> GSHMEAVQNRIVEAAERVPGVRGVIHLRARYVGQDIWADMIIGVDPENTVEQAEEICEAVQAAVCGKIRRIESLHVSAEAREIG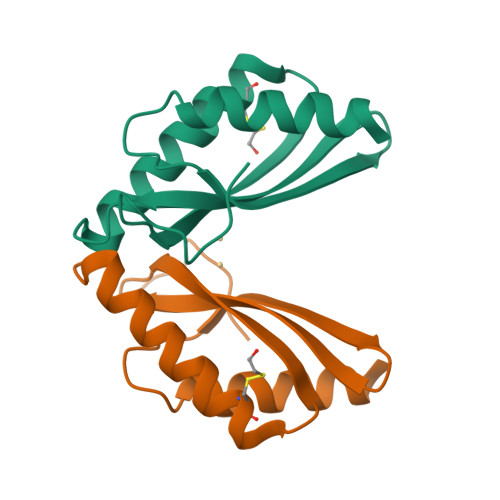DTTKPSFSDQPLSFDEVMLSKVDN> MSNEQTFIAIKPDGVQRGLIGPIISRFENRGFKLVAMKLVSPPQSQLEQHYADLSDKPFFKGLVSYMLSGPICAMVWEGRDVVKTGRTILGAT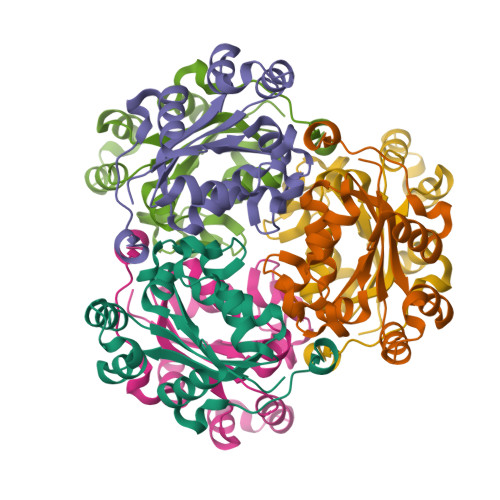NPLASAPGTIRGDFAIDVGRNVCHGSDSVENAKKEIALWFKPEELISWKSATFDWVYEKALEHHHHHH>[2x]SMVRRTKEEAQETRAQIIEAAERAFYKRGVARTTLADIAELAGVTRGAIYWHFNNKAELVQALLDSLHETHDHLARASESEDEVDPLGCMRKLLLQVFNELVLDARTRRINEILHHKCEFTDDMCEIRQQRQSAVLDIHKGWTLALANAVRRGQLPGELDAERAAVALYAYVDGLIRRWLLLPDSVDLLGDVEKWVDTGLDMLRLSPALRK

We chose TtgR, a ligand-inducible aTF belonging to the diverse TetR-like protein family, as a target for computational engineering of ligand specificity. TtgR is a 1-component transcriptional system and represents the simplest molecular mechanism for converting biophysical interaction between inducer and protein into a complex biological response like transcription. When induced, ligand-binding allosterically lowers affinity for DNA, thereby allowing transcription. TtgR is a compact, dimeric, all-helical transcription factor with a large cavity between five angled helices forming the ligand-binding pocket.

To understand the structural basis of TtgR-ligand interactions, we solved high-resolution crystal structures of quadruple mutant (resveratrol-bound and apo) and wild-type TtgR (resveratrol-bound) at a resolution of 1.9 Å or better. From the enriched population, we isolated a resveratrol-specific TtgR variant with four mutations: C137I, I141W, M167L, and F168Y which we will henceforth refer to as the ‘quadruple mutant’. All four mutations were in close proximity to the ligand and no mutations were found elsewhere on TtgR. The quadruple mutant gave 92- and 6.5-fold induction with 100 μM resveratrol and 1 mM naringenin, respectively, compared to 55- and 55-fold of wild-type TtgR. The DNA-binding domains of the resveratrol-bound quadruple mutant and the resveratrol-bound wild type are extremely similar with an all-atom RMSD of 1.0 Å. The four mutations do not substantially change the volume of the pocket (215Å3 in wild type compared to 234 Å3 in the quadruple mutant) or the surface area of the pocket (184 Å in wild type compared to 186 Å in the quadruple mutant). The biological effects of these mutations are further validated by the crystal structures. The four mutations localize to one face of the binding pocket, making nonpolar interactions with the ligand.> SY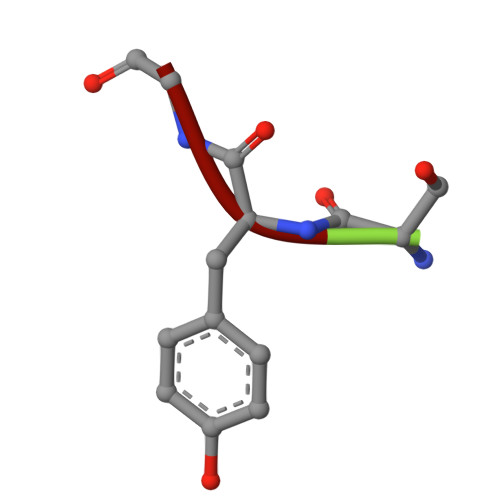G>MIFVNDVYKNFGSLEVLKGVTLKVNKGEVVVIIGPSGSGKSTLLRCINLLEEPTKGEVFIDGVKINNGKVNINKVRQKVGMVFQHFNLFPHLTAIENITLAPVKVKKMNKKEAEELAVDLLAKVGLLDKKDQYPIKLSGGQKQRLAIARALAMQPEVMLFDEPTSALDPEMVKEVLNVMKQLANEGMTMVVVTHEMGFAREVG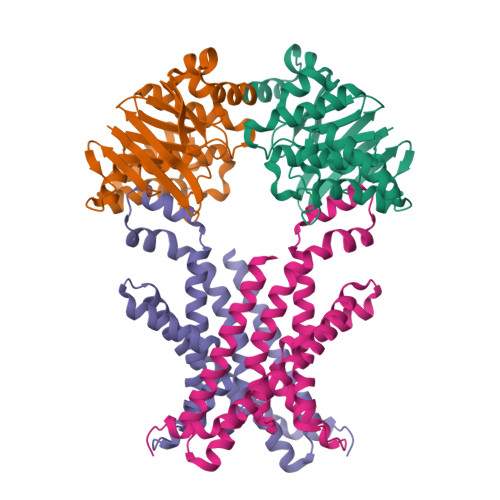DRVIFMDDGVIVEEGTPEEIFYRAKNERTREFLSKIL[2x];>[2x]MTVDFLSMVKYTPLFISGLIMTLKLTFLAVTIGVLMGLFIALMKMSSIKPIKLVASSYIEVIRGTPLLVQLLLIYNGLMQFGMNIPAFTAGVSALAINSSAYVAEIIRAGIQAVDPGQNEAARSLGMTHAMAMRYVIIPQAIKNILPALGNEFIVMLKESAIVSVIGFADLTRQADIIQSVTYRYFEPYIIIAAIYFVMTLTFSKLLSLFERRLRAGDIR>[3x]PPLDDPATDPFLVARAAADHIAQATGVEGHDMALVLGSGWGGAAELLGEVVAEVPTHEIPGFSSVTRSIRVE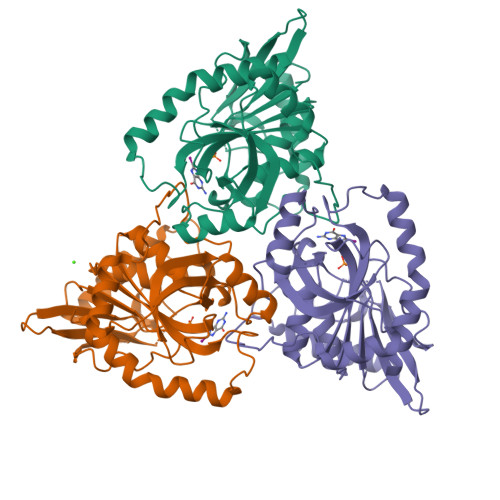RADGSVRHALVLGSRTHLYEGKGVRAVVHGVRTAAATGAETLILTNGCGGLNQEWGAGTPVLLSDHINLTARSPLEGPTFVDLTDVYSPRLRELAHRVDPTLPEGVYAQFPGPHYETPAEVRMAGILGADLVGMSTTLEAIAARHCGLEVLGVSLVTNLAAGISPTPLSHAEVIEAGQAAGPRISALLADIAKR~{N}-[4-(pyridin-4-ylmethyl)phenyl]benzenesulfonamide | C18 H16 N2 O2 S | 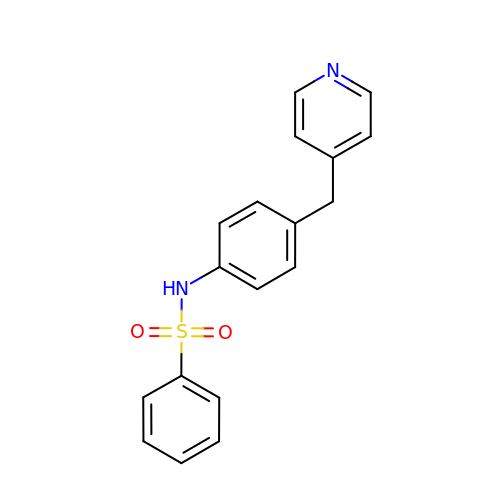CFLHYDJOEWYNKS-UHFFFAOYSA-N>SNAMTLNVIDSHFHIWDPDAQDLPWLAGLPSLQHRYTVDDLAAEYAKFGVNFLGGVYVEVDAADHELEDRLLYENASPLILKRMLQGRVSPWMRVPINADGIREPLHVDSEPRGRALEPEFIAGLRAMAAKGLPFELCNRGPELGDMAKAFAQVPEVTVIIDHLGNVPGLDEESCAALAALAELPNSYIKVSGDNPVGPDIVKYVRDTFGPKKVLYSSNWPVVELNSTFATHFQLMLDTFGEDEDFFENNARRAYNI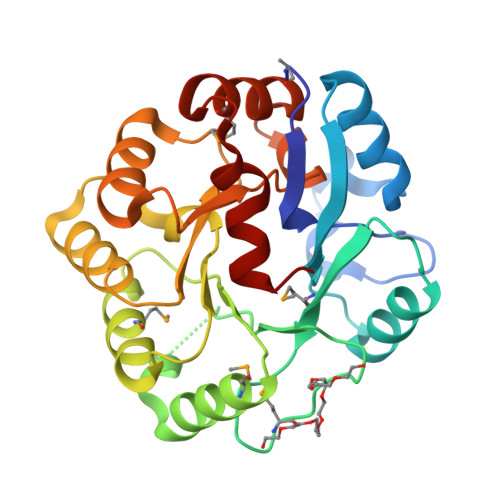D[5x]> ETAEPPGSPGAAATWTKGDKEGVGTSLNPASKVWYTLTEGTMSEVYYPHADTPNTRELQFAVSDGTSAQRESEQTTRTVELADPKALSYRQTTTDNAGRWRLTKTYVTDPRRSTVMLGVTFEVLDGGDYQLFVLSDPSLAGTSGGDTGSVTDGALLASDLADAATPVATALVSSVGFGAVANGYVGTSDGWTDLAADGRLDNASATAGPGNISQTGQIPLAAGGKTEFSLALGFGADTAEALATAKASLGTGYKKVSKSYTGEWKKYLNSLDAPATSLTGALRTQYDVSLMTVKSHEDKTFPGAFIASLTIPWGQAASAETHREGYHAVWARDMYQSVTALLAAGDEEAAARGVEWLFTYQQQPDGHFPQTSRVDGTIGQNGIQLDETAFPILLANQIGRTDAGFYRNELKPAADYLVAAGPKTPQERWEETGGYSTSTLASQIAALAAAADIAGKNGDAGSAAVYRATADEWQRSTEKWMFTTNGPVGDGKYYLRISATGNPNDGATRDWGNGAGVHPENAVLDGGFLEFVRLGVKAPADPYVADSLAETDASISQETPGGRMWHRYTYDGYGEKADGSPWDGTGIGRLWPLLSGERGEYALANGQDALPYLETMHSAANAGYMIPEQVWDRDEPTSYGHELGRSTGSASPLSWAMAQYVRLAAGVKAGAPVETPQNVAARYAAGTPLSSPELSVTAPEALSTADSATAVVRGTTNAAKVYVSVNGTATEAPVTDGTFSLDVALTGAKNKVTVAAVAADGGTAVEDRTVLYYGSRIGALSDPAGDDNGPGTYRYPTNSAYVPGAFDLTGVDVYDAGDDYAFVATIAGEVTNPWGGQAISHQRVNIYLGKGEGGATPGLPGTNINLEHAWDSVIVTDGRFDGAGVYAPDGTRTSAVSLLAVPEARQI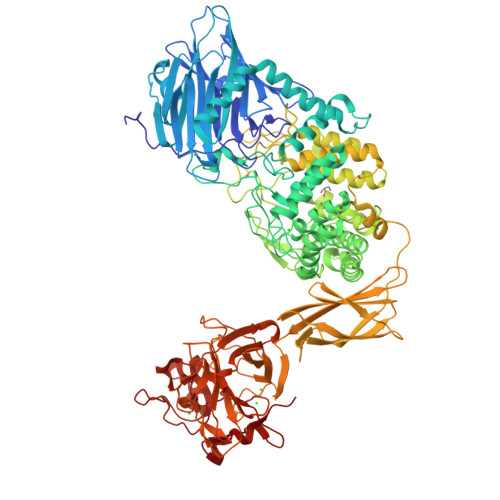VTRVPKAALGGLDPATARMSVAMFGNAESGEGIGNVRPVYDGAYWEAGDPAWIKEWRFGGGAGVFDGTIPSRDTDTDDPNALDVLVGEGQTQAAVLDWRAGSPVVVPMLGLQP>MQEAEYTLRLHHFFPASAPVHQEYFLPWKEAIEKESDGRLAVELYPSMQLGGTPPSLYDQAKDGQVDIIWTVLGYNSGRFPRAEVFDLPFLPTSGAATSQAAHEYAMTHMQDELEGVYPIAVHTHSPGALHTKETRIEALEDIEGLKMRGPSRLVNRYLAKLGAEPIGMPVAQALEALSRGVLDGTVIPFEAITAMGLADITTEHTIFSGDRALYTTMMIVAMDQDKYDALPEDLQPIIDAHAGGREAYRIG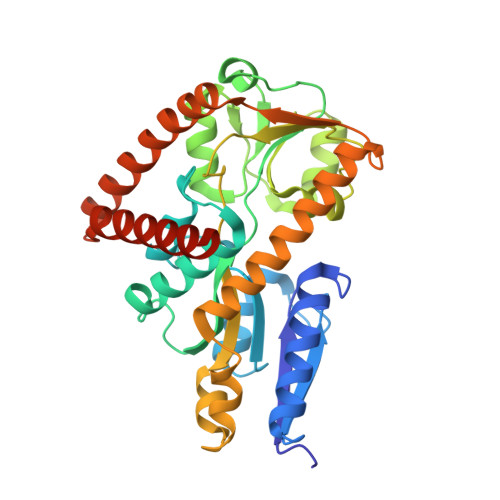QIMDQADHRQILAIQSGEQPGTITRLGSEETARWQAVGQEVVDEWIAEAEEKGLDGQMLYDDATRLVERYTRAAALEHHHHHH[2x]>SGTATYSGNPFVGVTPWANAYYASEVSSLAIPSLTGAMATAAAAVAKVP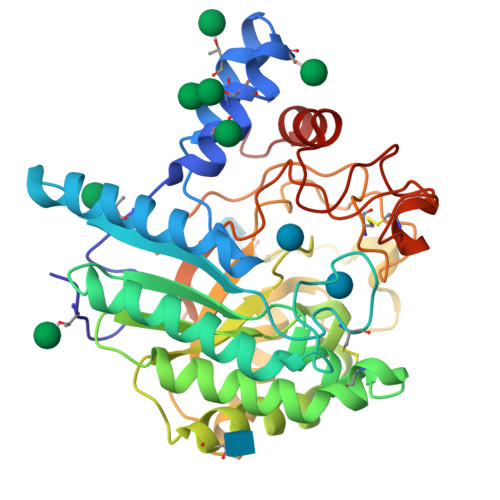SFMWLDTLDKTPLMEQTLADIRTANKNGGNYAGQFVVYDLPDRDCAALASNGEYSIADGGVAKYKNYIDTIRQIVVEYSDIRTLLVIEPASLANLVTNLGTPKCANAQSAYLECINYAVTQLNLPNVAMYLDAGHAGWLGWPANQDPAAQLFANVYKNASSPRALRGLATNVANYNGWNITSPPSYTQGNAVYNEKLYIHAIGPLLANHGWSNAFFITDQGRSGKQPTGQQQWGDWCNVIGTGFGIRPSANTGDSLLDSFVWVKPGGECDGTSDSSAPRFDSHCALPDALQPAPQAGAWFQAYFVQLLTNANPSFL[2x]6-{[(3R,4R)-4-(2-{[2-(2-chlorophenyl)-2,2-difluoroethyl]amino}ethoxy)pyrrolidin-3-yl]methyl}-4-methylpyridin-2-amine 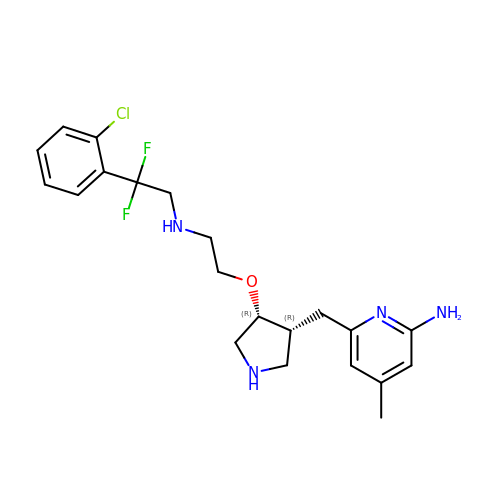| C21 H27 Cl F2 N4 O | JVSYUOBMDVYGPZ-BEFAXECRSA-N>[2x]MGSSHHHHHHSQDPSKTGADKGLSNLCEGIANALFPPSIQATIASGSKKVLTNNKPAARAAGIAPPTQISGDGAEEGEATDTPSATPEEGPGFLDMAKEFFSQMWRPTVASPAPGSQTKELDLVTCTKHPPMPVQYLAEGSEKVSIDGQPAVRSGDRSTCDAKVVSAGPISPNVTIGGGSVVVREIRSGKTPGVGLAVTVLMMLKGGKGKFLSNLPCMLMAGVNSFVVSQATNALTQAVVASTHPVHAATGAKVLGADDDLDFTLPGLMPIEWQRFYNSRDERRDGLLGAGWSLPYEISVQIEPHPEGGERLLYIDEQGRRIDMGSIALGAGAFSPGEGLSVRRNENGQLLIESSDGIYRLF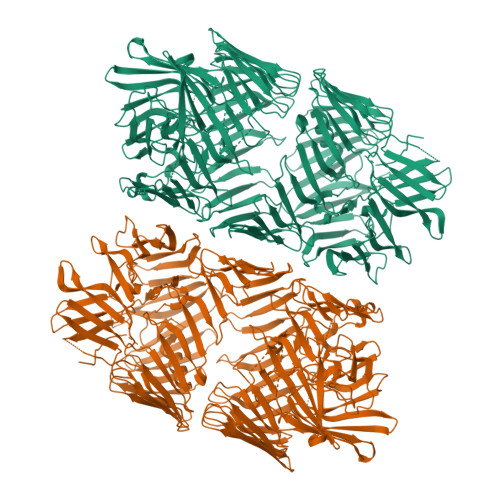EPLPGDSSRLRLSLLGDRNDNRLHLEYDSSGRLWLLRDTFEQAQLELSYSTLWPGRIAQVERLYPDQQREVLVSYDYDAAGDLAQVRDSEGQVQRRFAYDAGHRMIEHQLATGLRCFYQWTQFADQQWRVTRHWTDEGDSYQYDYDLEAGITQVTDSLQRLSRRRWNSQLQIVEYTDNLNQTWAFEWNDERQLLSATDPLGGRYAYSYDETGNLIAETDPLGHSHSTLWLEHWSLPQTLTDPAGESWHLRYDPRGNCIAEVDPLGQVTQYRHDAHGQVVEIIDAAGRSRKMRWNSSGQLLEHLDCSGYPTRFEYDRRGNVKAIIDALGEHTRFHYDCQGRLLSSQLADGRAEHFQRSSNGQLQGYTDPSGYTTLYQYNRRGQIRQRIDAHGRQVRFDYDAYGRLLALTNENGESYRFAWDAGNRLSEQQDLDGSAKRYGYDLLNNVVELQSHPAPYGTGLSAVPAQPIAPIIHRFERDAVGRLLAKITDDGRSQYTYDPLNQLTAASFTDNLGNQQALSFSYDALGQLLEEHTVAGSLIHRYDELGNLTQTQLPDKRWLNRLYYGSGHLHQINLDGQVVSDFQRDRLHREVLRTQGQISTRSEYDRCGRLRARLQHSSLLANTLPTAPERHLEYDDSDNLVGLAERHATGQHRQLFHYDATGRIIASQDGLQGQKETFAYDAAANLLDGPKAGAGLVVHNKLLTYQDKRYRYDAFGRMIEKRSGRRGVQRFAYDAEHRLIEVRNQTSSGETLVRMRYDVLGRRISKSEYDSQGNLLGETRFVWDGLRLLQEQRNQQTSLYVYEDLGHAPLARVDGLGAQQKIRYYHNDLNGLPQQLCEPDGHSVWQARYQVWGNTVEEIREPYYIEEQNLRFQGQYLDRETGLHFNTFRFYDPDIGRFTTPDPIGLAGGLNLYQYAPNPIGWIDPLGWICKSAYSGRRGTTKAKADLERNGFTVVGEELTMKVKHPVTQKSYRIRADIIAKDKAGNYHVFEVKNGSGKLTKNQQGSGMFDMSNPANTNGGLGGGLIKPSGATQGQFEVATKTARGTQFGGNGAQHSATFWLLRY> GSHMKQSFRDNLKVYIESPESYKNVIYYDDDVVLVRDMFPKSKMHLLLMTRDPHLTHVHPLEIMMKHRSLVEKLVSYVQGDLSGLIFDEARNCLSQ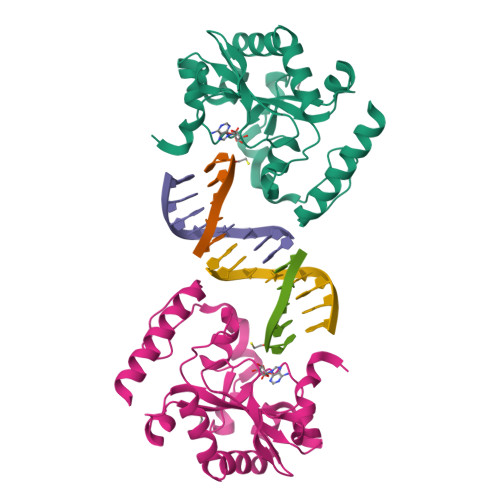QLTNEALCNYIKVGFHAGPSMNNLHLHIMTLDHVSPSLKNSAHYISFTSPFFVKIDTPTSNLPTRGTLTSLFQEDLKCWRCGETFGRHFTKLKAHLQEEYDDWLDKSVSM> GPLGSMSQSNRELVVDFLSYKLSQKGYSWSQMAAVKQALREAGDEFELRYRRAFSDLTSQLHITPGTAYQSFEQVVNELFRDGVNWGRIVAFFSFGGALCVESVDKEMQVLVSRIASWMATYLNDHLEPWIQENGGWDTFVELYGN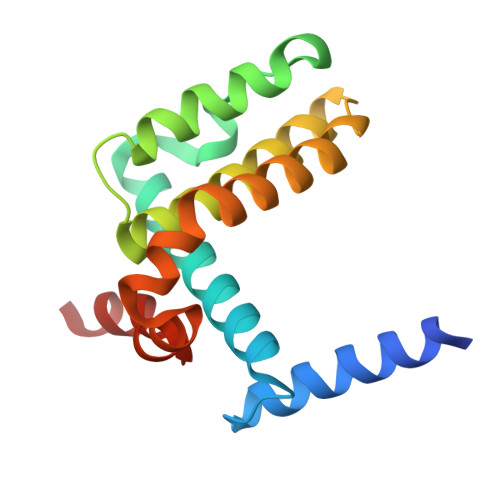NAAAESRKGQER> GMQSWSAPAIPVVPGRGPALRLFDSADRQVRPVTPGPTATMYVCGITPYDATHLGHAATYLTFDLVHRLWLDAGHTVQYVQNVTDVDDPLFERAERDGIDWRTLGDRETQLFREDMAALRVLPPHDYVAATDAIAEVVEMVEKLLASGAAYIVEDAEYPDVYFRADATAQFGYESGYDRDTMLTLFAERGGDPDRPGKSDQLDALLWRAERPGEPS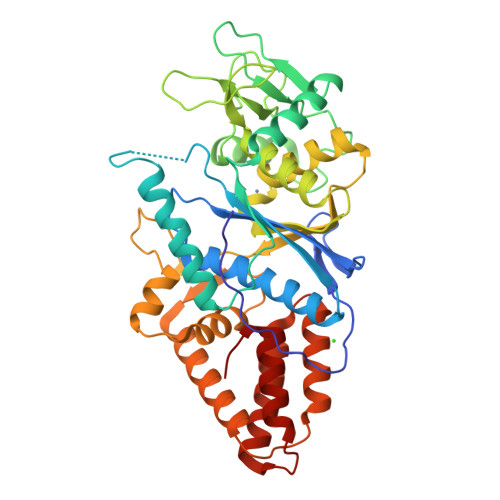WPSPFGRGRPGWHVECSAIALTRIGTGLDIQGGGSDLIFPHHEYSAAHAESVTGERRFARHYVHTGMIGWDGHKMSKSRGNLVLVSQLRAQGVDPSAIRLGLFSGHYREDRFWSNEVLDEANARLARWRSATALPEAPDATDVIARVRQYLADDLDTPKALAALDGWCTDALSYGGHDTESPRLVATTVDALLGVDL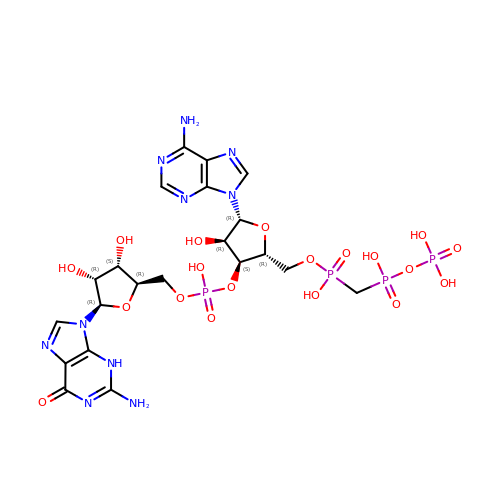[(2R,3S,4R,5R)-5-(6-aminopurin-9-yl)-3-[[(2R,3S,4R,5R)-5-(2-azanyl-6-oxidanylidene-3H-purin-9-yl)-3,4-bis(oxidanyl)oxolan-2-yl]methoxy-oxidanyl-phosphoryl]oxy-4-oxidanyl-oxolan-2-yl]methoxy-[[oxidanyl(phosphonooxy)phosphoryl]methyl]phosphinic acid | C21 H30 N10 O19 P4 | QFHKDAVOJDVDDK-XPWFQUROSA-N>[4x]MPVAGSELPRRPLPPAAQERDAEPRPPHGELQYLGQIQHILRCGVEKDDRTGTGTLSVFGMQARYSLRDEFPLLTTKRVFWKGVLEELLWFIKGSTNAKELSSKGVKIWDANGSRDFLDSLGFSTREEGDLGPVYGFQWRHFGAEYRDMESDYSGQGVDQLQRVIDTIKTNPDDRRIIMCAWNPRDLPLMALPPCHALCQFYVVNSELSCQLYQRSGDMGLGVP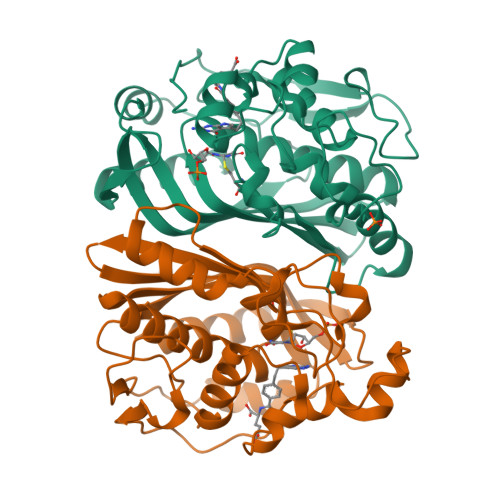FNIASYALLTYMIAHITGLKPGDFIHTLGDAHIYLNHIEPLKIQLQREPRPFPKLRILRKVEKIDDFKAEDFQIEGYNPHPTIKMEMAV> GAMAAGTLYTYPENWRAFKALIAAQYSGAQVRVLSAPPHFHFGQTNRTPEFLRKFPAGKVPAFEGDDGFCVFESNAIAYYVSNEELRGSTPEAAAQVVQWVSFADSDIVPPASTWVFPTLGIMHHNKQATENAKEEVRRILGLLDAYLKTRTFLVGERVTLADITVVCTLLWLYKQVLEPSFRQAFPNTNRWFLTCINQPQFRAVLGEVKLCEKMAQFDA;> GAMGFGDLKSPAGLQVLNDYLADKSYIEG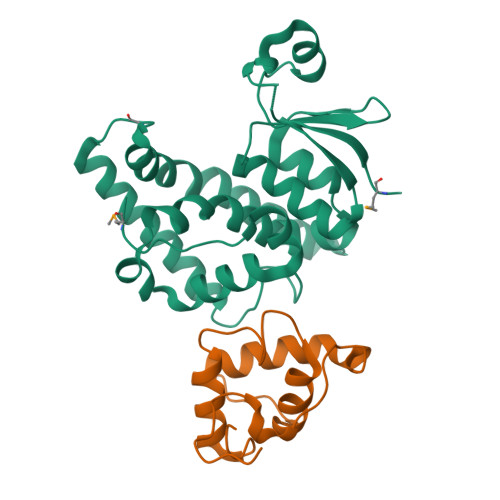YVPSQADVAVFEAVSSPPPADLCHALRWYNHIKSYEKEKASLPGVKKALGKYGPADVEDTT Enzymes of the vanillyl alcohol oxidase/p-cresol methyl hydroxylase (VAO/PCMH) superfamily are found across all kingdoms where they perform a range of metabolic functions. These flavoproteins share a conserved FAD-binding domain and a more variable substrate-binding domain that enables interactions with a range of substrates. One of these, the 4-phenol oxidases/dehydrogenases, catalyzes the oxidation of para-substituted phenolic compounds. A fundamental distinction is that the oxidases efficiently react with oxygen producing hydrogen peroxide whereas the dehydrogenases hardly react with oxygen and typically employ other proteins, such as cytochrome c, as acceptors.

Pro151 was substituted with isoleucine and valine to mimic the N5 environment of EUGHs. We found that P151V and P151I can operate with oxygen although they are 10- to 40-fold less efficient compared to using 2,6-dichlorophenolindophenol as co-substrate. The crystal structures of the six P151 mutants were also solved. They are closely similar to the wild-type regarding the substrate-binding residues whereas loop 150-153 locally undergoes localized rearrangements, with each mutant adopting a distinct conformation. In general, the oxidase-active variants (P151L, P151G, P151I, P151V) all adopt the trans conformation that slightly shifts the amino acid at position 151 away from the flavin. The analysis revealed a consistent pattern: in the oxidase mutants, the 150-153 loop conformations create tunnels that lead to the flavin re side.

>[2x]MAAPLPEGVSAEAMSSALDRFARIVGADWVFTEDKITPYEDPYTISNDETEHRPYAAVAPASTEEVQEIVRVANEFGVPLWPVSRGKNFAYGGAAPVMSGTVVLDMNRMNRILEVNEEFGYALVEPGVSYFELYDYIQEKGLKLWIDVPDIGWGSVVGNALDHGIGYTPYGDHFAMQCGMEVVLPNGEVVRTGMGAMPGNNTWQLFKYGYGPYVDGIFSQSNFGVVTKMGIWLMPEPAGYRPYLITFENEDDIETVTERLRPLKVAGVIQNGATVRSLVLDAAITRTKSQYYDGDGPIPPSVAKTMMADLDLGMWNFCGALYGPPPVMDTLWTAIRDSFADIPGVKFYFPEDRRHKVDLLLHRAETMKGVPKLTEFNFLNWDGGGGHVGFSPVSPITGKDAIKQYNMVSSRVREYGFDYMGLLAIGWRDLHHVTVIVYDKTDPDERKKLDELFNILVDEAAAEGYGEYRTHIRYMDRIAKTYSWNDNALWKMHETIKDALDPNGILAPGKSGIWGKNRRKA>EHEHNYHPNAVAAGLRAGRTRSIGLVIPDLENTSYTRIANYLERQARQRGYQLLIACSEDQPDNEMRCIEHL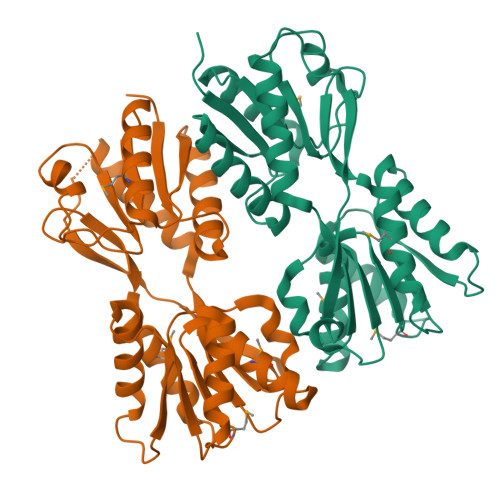LQRQVDAIIVSTSLPPEHPFYQRWANDPFPIVALDRALDREHFTSVVGADQDDAEMLAEELRKFPAETVLYLGALPELSVSFLREQGFRTAWKDDPREVHFLYANSYEREAAAQLFEKWLETHPMPQALFTTSFALLQGVMDVTLRRDGKLPSDLAIATFGDNELLDFLQCPVLAVAQRHRDVAERVLEIVLASLDEPRKPKPGLTRIKRNLYRRGVLSRS[2x]>[2x]MEHRHLKPFPPEFLWGAASAAYQVEGAWNEDGKGLSVWDVFAKQPGRTFKGTNGDVAVDHYHRYQEDVALMAEMGLKAYRFSVSWSRVFPDGNGAVNEKGLDFYDRLIEELRNHGIEPIVTLYHWDVPQAL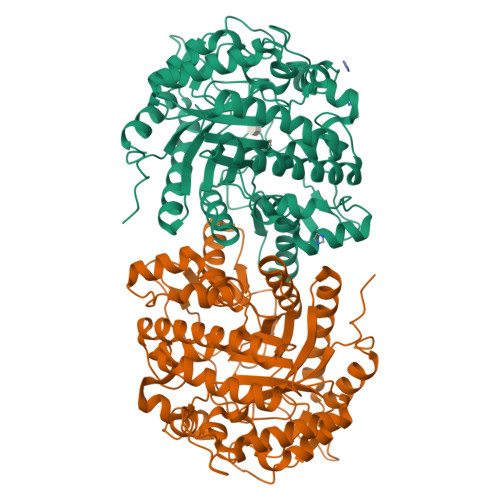MDAYGAWESRRIIDDFDRYAVTLFQRFGDRVKYWVTLNEQNIFISFGYRLGLHPPGVKDMKRMYEANHIANLANAKVIQSFRHYVPDGKIGPSFAYSPMYPYDSRPENVLAFENAEEFQNHWWMDVYAWGMYPQAAWNYLESQGLEPTVAPGDWELLQAAKPDFMGVNYYQTTTVEHNPPDGVGEGVMNTTGKKGTSTSSGIPGLFKTVRNPHVDTTNWDWAIDPVGLRIGLRRIANRYQLPILITENGLGEFDTLEPGDIVNDDYRIDYLRRHVQEIQRAITDGVDVLGYCAWSFTDLLSALNGYQKRYGFVYVNRDDESEKDLRRIKKKSFYWYQRVIETNGAEL N-HEXYLPHOSPHONATE ETHYL ESTER | C8 H19 O3 P | 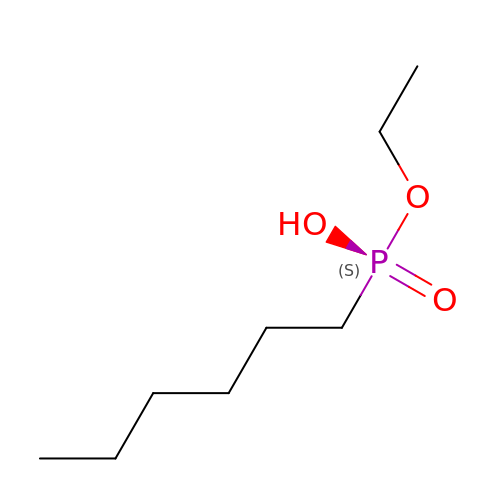XPLOQMVUXWZLET-UHFFFAOYSA-N>[2x]MGSSHHHHHHSQDPNSMTAQLASHLTRALTLAQQQPYLARRQNWVNQLERHAMMQPDAPALRFVGNTMTWADLRRRVAALAGALSGRGVGFGDRVMILMLNRTEFVESVLAANMIGAIAVP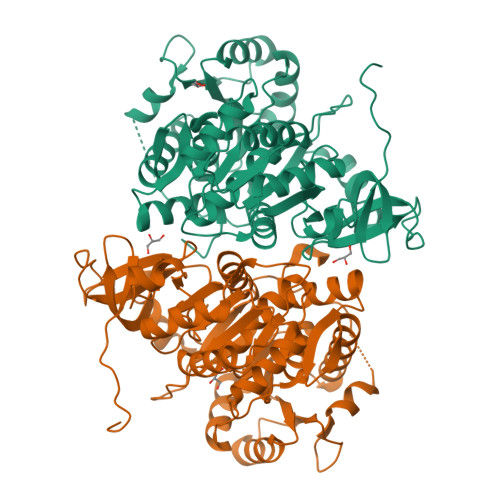LNFRLTPTEIAVLVEDCVAHVMLTEAALAPVAIGVRNIQPLLSVIVVAGGSSQDSVFGYEDLLNEAGDVHEPVDIPNDSPALIMYTSGTTGRPKGAVLTHANLTGQAMTALYTSGANINSDVGFVGVPLFHIAGIGNMLTGLLLGLPTVIYPLGAFDPGQLLDVLEAEKVTGIFLVPAQWQAVCTEQQARPRDLRLRVLSWGAAPAPDALLRQMSATFPETQILAAFGQTEMSPVTCMLLGEDAIAKRGSVGRVIPTVAARVVDQNMNDVPVGEVGEIVYRAPTLMSCYWNNPEATAEAFAGGWFHSGDLVRMDSDGYVWVVDRKKDMIISGGENIYCAELENVLASHPDI> SRQGSTQGRLDDF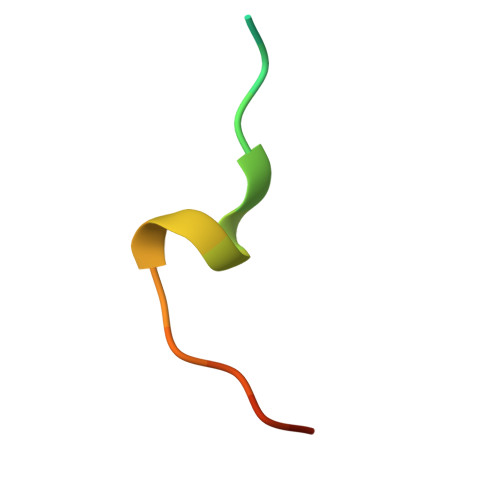FKVTGSL> GKMLVVYMTLGYPNVQSFKDFIIGAVENGADILELGIPPKYAKYDGPVIRKSYDKVKGLDIWPLIEDIRKDVGVPIIALTYLEDWVDQLENFLNMIKDVKL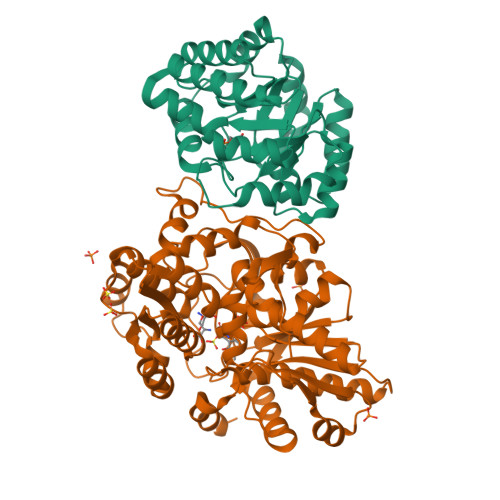DGILFPDLLIDYIDDLDKIDGIIKNKGLKNVIFTSPSVPDLLIHKVSKISDLFLYYGVRPTTGVPIPVSVKQLINRVRNLVENKLIVGFGLSSESDLRDALSAGADGIAIGTVFIEEIERNGVKSAINLVKKFRAILDEY;> MVKEDEILPKYWYNIIPDLPKPLPPPRDPQGAYFSRIDLLRSILPKEVLRQQFTIERYIKIPEEVRDRYLSIGRPTPLFRAKRLEEYLKTPARIYFKYEGATPTGSHKINTAIPQAYFAKEEGIEHVVTETGAGQWGTAVALAASMYNMKSTIFMVKVSYEQKPMRRSIMQLYGANVYASPTNLTEYGRKILETNPQHPGSLGIAMSEAIEYALKNEFRYLVGSVLDVVLLHQSVIGQETITQLDLLGEDADILIGCVGGGSNFGGFTYPFIGNKKGKRYIAVSSAEIPKFSKGEYKYDFPDSAGLLPLVKMITLGKDYVPPPIYAGGLRYHGVAPTLSLLTKEGIVEWREYNEREIFEAAKIFIENQGIVPAPESAHAIRAVVDEAIEARKNNERKVIVFNLSGHGLLDLSNYESMMKRLNGNG2-({4-[(2-amino-4-oxo-4,7-dihydro-3H-pyrrolo[2,3-d]pyrimidin-5-yl)methyl]benzene-1-carbonyl}amino)-4-cyanobenzoic 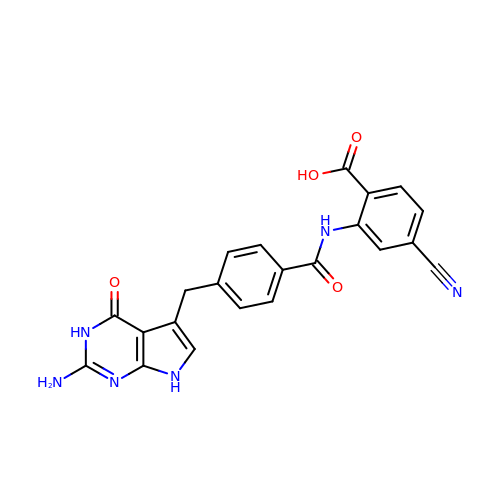acid | C22 H16 N6 O4 | MEWIMDIPLNOYGN-UHFFFAOYSA-N> MQTQEVAIKPNLKVVLRSDAQQIDEVVVTAMGIKRSEKALGYAATSVGGEKIAESRTSDVMSSLAGKIAGVQISSTSSDPGASNSVIIRGVSSLSGTNQPLYVVDGVPLNNSTVYSTDGLNSGYDFGNGANAINPDDVANMTILKGAAATALYGSRAANGVVMITTKSGRKEKGVGIEY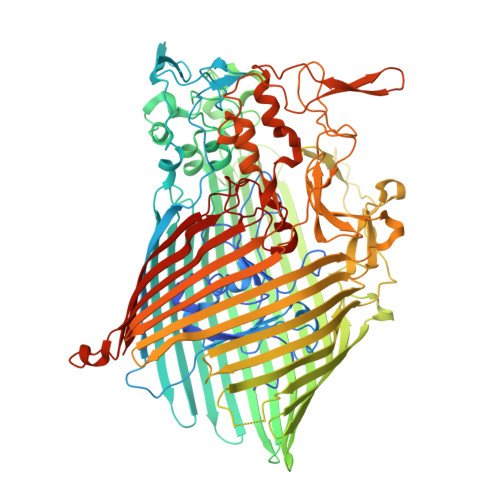NGGVQWSTVLRLPEFQNEFGMGWNGNHTELENGSWGPRFDGSMQLWGNVYNNSQKLKPYVAMPDNIKDFFDAGFRYSNSLSFNGATDKSDYYVSFSQISDDGMIPTDADSYDKYTFSARGSHKAGALTFSSSLNYAYQKNNFATTGQGLSMLNSLYQTPRDISIIGLEDQNDPFNTPGYYYTPYGVMNPYYILNNYLNEYESERFYGKFQLDYEFLKYFKFTYRMGLDTTTGQSDKGKPNLYALYYEGTPNGEGQGSSSPFSGETGQYSEQITRRREINQDIMVNFNMPVNDFNINALVGFNGNERKVSYQYSEVNDLTIPTWFNLKNSGKTPIVEQHMELRRLMGVFGQFEGSWKNMLYLTVTARNDWSSTLPKENRSFFYPGITGSFIFSELLNDNLQDVITFGKIRASWGKTGNDADVYMVNPVYAQSSNRIPFGSLTFPLGGVNAYSAGNVLGSNTLSPEMTTESEVGLNMAFFKNRLSFDVSYYNRNTDKQIFSLAMDPASGYTAQNMNLGKIRNRGIELLISGTPIRTKDFSWELTWNFTKNWSKVISLPEELGGITTIYGLNGGTSMYAITGMPVGVFKAQVAERDPQGRIVVNSSTGLPVEASEFGICGDMNNKYQMGVSTNLKYKGISLGIDFDIRQGGVMYSRTKDINYFTGNAIQTAYNDRNPLIVPNSVNKIVNGENVTYVENTTPITSSNIYKYWGDGGSDMGSCFLVDKSYVKLRSVVLGWDLPKRWLAKTPFQAVKVSAYGNNLFVWTPSSNTFIDPEMTSFGNDLEGNYGEYTANPSSRRFGFNLMVKF> GAGCAGACCTG;> ACGACACTCA;> CACGT;> T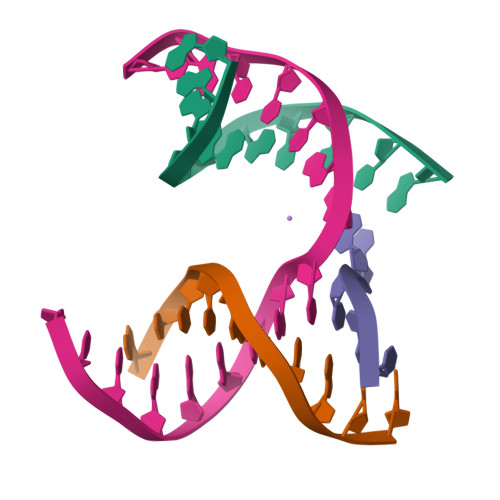CTGAGTGTGGTCTGC> MLAKRIIACLDVKDGRVVKGTNFENLRDSGDPVELGKFYSEIGIDELVFLDITASVEKRKTML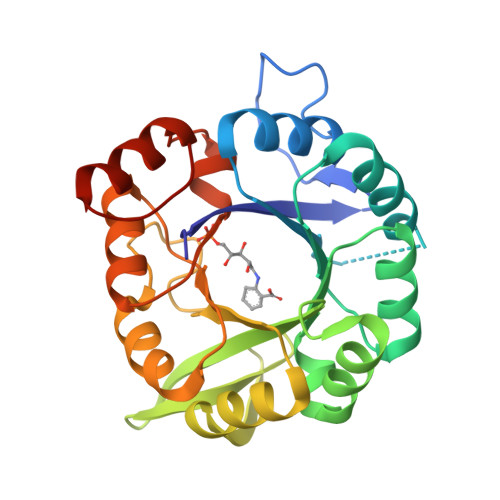ELVEKVAEQIDIPFTVGGGIHDFETASELILRGADKVSINTAAVENPSLITQIAQTFGSQAVVVAIVAKRVDGEFMVFTYSGKKNTGILLRDWVVEVEKRGAGEILLTSIDRVGTKSGYDTEMIRFVRPLTTLPIIASGGAGKMEHFLEAFLAGADAALAASVFHFREIDVRELKEYLKKHGVNVRLEGL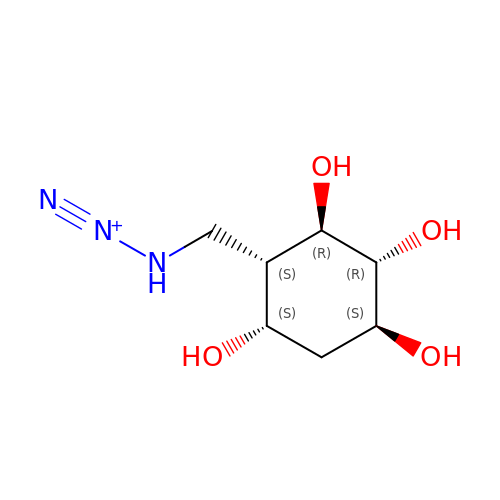(1~{S},2~{R},3~{R},4~{S},5~{S})-4-[[($l^{5}-azanylidyne-$l^{5}-azanyl)amino]methyl]cyclohexane-1,2,3,5-tetrol | C7 H14 N3 O4 | FBFTWYYGVGMNEW-YPPKRKOXSA-N Eukaryotic initiation factor 4E (eIF4E) serves as a regulatory hub for oncogene-driven protein synthesis and is considered a promising anticancer target. The eIF4F complex includes a core of eIF4E, eIF4G and eIF4A5,6. eIF4E recognises and binds the mRNA 5’cap, and recruits eIF4G to provide a scaffold function for the eIF4F complex, while eIF4A is an RNA helicase that is stimulated by binding to eIF4E and eIF4G8. Here we screen a fragment library against eIF4E and identify a ligand-binding site with previously unknown function.

Compound 2 bound in a similar region to 1 but caused elongation of the α1-helix and movement of the loop region (consisting of residues 80–86 between the α1-helix and β3-sheet) resulting in a larger more solvent exposed binding site. The loop is mobile with high B-factors and incomplete density for several residues. The cyclopentyl-carboxylic acid occupies the region of L81 and S82 in the compound 1 structure, displacing a water molecule (W2) observed in the crystal structure of 1, making interactions with Q80 S83, N127 and Y76. The affinity of this fragment was much weaker, Kd = 7400 µM with low ligand efficiency (LE 0.19), possibly related to the energetic penalty paid for inducing the change in protein conformation and/or inadequately filling the hydrophobic binding site. Compound 2 binds in close proximity to the non-canonical binding region of eIF4G / 4E-BP described by both Sekiyama50 and Gruner51.

>[2x]MHHHHHHGARIIYDRAFLMACRGGGGENLYFQGKHPLQNRWALWFFKNDKSKTWQANLRLISKFDTVEDFWALYNHIQLSSNLMPGCDYSLFKDGIEPMWEDEKNKRGGRWLITLNKQQRRSDLNRFWLETLLCLIGESFDDYSDDVCGAVVNVRAKGDKIAIWTTECENREAVTHIGRVYKERLGLPPKIVIGYQSHADTATKSGSTTKNRFVV> GSAHGPSAMVFTVIQGSGEPTDTVLRATTLSCAYT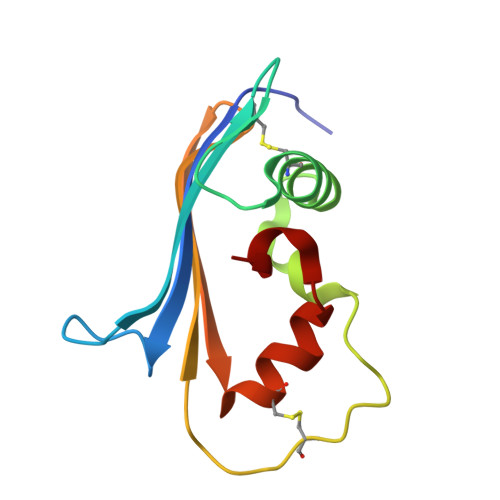AEGTHPAPRAACDALNATDGELNRLLAAPDPSLVCPMYFDPVTVTADGVLNGRRVAWKHTFSNTCVMSANLNSNPVYAF Rhodopsins mediate passive or active ion transport or metabotropic reactions in response to light and share a common architecture, consisting of a single polypeptide with 7-transmembrane (7TM) segments (opsin) and a retinal chromophore covalently attached to a conserved lysine residue via a Schiff base. ChRs mediate phototaxis in green algae and are exceptionally popular in neurosciences, where they are used to manipulate neuronal activity with light to study multiple aspects of brain function ranging from synaptic plasticity to network analysis. More recently, a ChR from Chlamydomonas noctigama (Chrimson) was identified as the variant with the most red-shifted absorption peak at 590 nm, which is more than 40 nm further red-shifted than all other ChRs. Therefore, Chrimson represents one of the most promising ChRs for both basic neuroscientific research and medical applications.

Here we present the crystal structure of Chrimson at 2.6 Å resolution, which reveals (i) the presence of an outer gate occluding the retinal Schiff base from the extracellular solvent, (ii) unique protonation state of the counterion residue destabilizing the protonated retinal Schiff base in the ground state, (iii) highly biased polar residue distribution toward the β-ionone ring, and (iv) tight association with the retinal chromophore to improve the retinal planarity, which appears essential for fast photocycle kinetics. As the expression level of wild-type Chrimson is very low in insect cells, we tested two Chrimson variants in which the extracellular N-terminal sequence was replaced by either the corresponding sequence of the Chloromonas subdivisa channelrhodopsin (CsChrimson) or the N-terminal sequence of CrChR1 (C1Chrimson). The two protomers in the asymmetric unit form a dimer, with each protomer composed of the extracellular N-terminal domain, 7TM helix bundle and the C-terminal β-hairpin loop region. The CrChR1-derived N-terminal residues mediate the crystal packing contacts between the layers in the lipidic cubic phase crystal and facilitate the dimeric interaction by forming the inter-protomeric β-sheet and three disulfide bonds. Although Chrimson is distantly related to the CrChRs (about 50% sequence identity over transmembrane region), the overall structure of Chrimson superimposes well with those of C1C2. In the current ground state structure of Chrimson, the ion-conducting pore is closed by three constriction sites that restrict ion permeation, on the intracellular side (inner gate), at the middle of the membrane (central gate), and on the extracellular side (outer gate). In Chrimson, direct hydrogen bonding between Glu139, Tyr159, and Ser288 interconnects TM2, TM3, and TM7 and constitutes the outer gate constriction. The crystals of Chrimson were obtained under low pH conditions, and the blue color of the crystals indicates that the current structure represents its red light-absorbing (protonated) state.

>MSRRPWLLALALAVALAAGSAGASTGSDATVPVATQDGPDYVFHRAHERMLFQTSYTLENNGSVICIPNNGQCFCLAWLHSRGTPGEKIGAQVCQWIAFSIAIALLTFYGFSAWKATCGWEEVYVCCVEVLFVTLEIFKEFSSPATVYLSTGNHAYCLRYFEWLLSCPVILIKLSNLSGLKNDYSKRTMGLIVSCVGMIVFGMAAGLATDWLKWLLYIVSCIYGGYMYFQAAKCYVEANHSVPKGHCRMVVKLMAYAYFASWGSYPILWAVGPEGLLKLSPYANSIGHSICDIIAKEFWTFLAHHLRIKIHEHILIHGDIRKTTKMEIGGEEVEVEEFVEEEDEDTV[2x]> DAVVVTGYQTVERRKLTAAVGKLNISDETIGAVKSIDQALAGQIAGLSVTSTSGAPGAPAKIRIRGTSSLNGTQDPLWVLDGIPLEGTDVPQSNVLNDVSNIQQSSIAGLNPADIENITVLKDAAATAIYGARAANGVIVITTKKGKVGKPVINFSSKFTYMPTLSTNRLNMLNSQEKVDLELELLRSNFAYGDNKGGVSKIISGYGLTDAYKKGGWSALTPEAQTDISRLRNTETDWGDILFRDAFNQEYSLSLSGGNERVTYYTSIGYYQENGNVKGVGLDRLNIVAKTSYKVN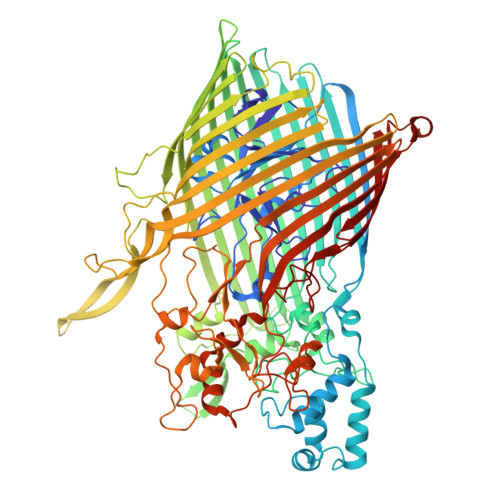RMLKFGVSLFVNRRNNKTYLTDTYGLVNPVYYSRKANPYYQPFDANGNYVYDFDVQNNSDTDLGFNIFEERKNTSNEETINALSSIFDAELRFNDKLKFTTQLGLQLDKASKEQIADKESFSMRIIRKNSKYWDSASQSNKYFIPDGGVHKAYENTNSQITWKAMGEYRDSFNDIHELEVMVGTELRKTWYETLFSAGYGFDRQTLTTKPVVFPDEDRARQFPLHQKTYKENAYVSFFSTASYSLMNRYTFGGSIRFDGSDLFGVDKKYRYLPLYSVSGLWRLSNEPFMQGTRKWMDNLAFRVSYGIQGNIDKNTSPFLLGKYIVDNILPGGSEHMIDINSAPNKKLRWEKTQSVNVGLDFSVLNQALNLSVDYYYRKGTDLIGKQMLPLETGFVSTNINWASMVNKGVEVSLSTRNVATKNFSWYTNLNFAYNNNKVLREAIPEAQTIPGREGYPVDAIFAIKTAGLDEEGYPLFYDKEGKKVTLKELYRLQDPFGLGFTVNSDVTPAEERSFYSYIGSQDTPYTGGLINTFSYKNWELTANLSFNLGGYVRTTPSYNFINFDRGQNVNSDILDRWTPENTDGRLPALITSEKRADEYYWYDQKSEIYKNLDIWVKKLNYFRLQNLRLGYRLPEKMTKSLGMGSASVAIEGRNLLVFGSSYKNFLDPESMYNPYAPPIPKSITFSLNLNF Iodothyronine deiodinases (Dio) are selenocysteine-containing membrane enzymes that activate and inactivate the thyroid hormones (TH) through reductive iodide eliminations. The three deiodinase isoforms are homodimers sharing highly conserved amino acid sequences, but they differ in their regioselectivities for the deiodination reaction and regulatory features. Dios feature homologous transmembrane regions and catalytic domains with a catalytic selenocysteine (Sec) residue essential for their unique reductive deiodination mechanism. The Dio isoforms differ, however, in their regioselectivities: Dio1 can catalyze deiodination of both the inner (tyrosyl) and the outer (phenolic) ring, while Dio2 targets only the outer ring and Dio3 only the inner ring.

To explore the molecular basis of deiodinase isoform differences, we solved a crystal structure of the catalytic domain of Mus musculus Dio2 (mDio2cat; residues 71–262). The catalytic Sec130 was replaced with cysteine to simplify bacterial overexpression. Two lysine residues, Lys180-Lys181, were predicted as the best SER candidates based on sequence analyses with the SERp server and consistent with the structure of the homolog mDio3cat (likely surface position) and were thus mutated to Ala. The protein mDio2cat-(Lys180Ala-Lys181Ala; mDio2cat-AlaAla) indeed formed well-diffracting crystals and the structure of mDio2cat-AlaAla (from now on referred to as mDio2cat) could be solved and refined at a resolution of 1.1 Å to R/Rfree values of 14.5% and 16.9%, respectively. The mDio2cat structure comprises 183 residues, covering an N-terminal Gly as a cloning artifact, a small part of the linker to the transmembrane region (71–76), and the complete catalytic core (77–261), except for the C-terminal Arg262 and residues 94–102, which are not defined by electron density. All residues of the structure are within favored (96.5%) or allowed regions (2.9%) of the Ramachandran plot, except for Phe224, which is well defined by electron density. mDio2cat features a Trx/Prx fold with deiodinase-specific modifications and insertions and high similarity in the overall structure to mDio3cat, confirming the proposed conservation of a Trx/Prx-related fold among the Dio isoforms. The basic Trx fold provides β-strands β1–4, and the sheet they form is extended by a single strand, βD, from the deiodinase-specific insertion that further comprises an α-helix αD and the extended loop-D (residues 161–188), which protrudes out of the globular structure. A major difference between Dio2 and other isoforms, however, is a 15-residue (91–105) “Dio2-insertion” in the N-terminal region of the catalytic core. Interestingly, there is no electron density for nine central residues of the Dio2-insertion (94–102), indicating conformational heterogeneity or high flexibility.

> GAYKQVKLGEDAPNSSVVHVSNPESGNNYASEKTADGAECHLLDFASAERPLVVNFGSATCPPFTRQLPAFRQLVEEFSSVADFLLVYIDEAHPSDGWAVPGDSSLSFEVAAHRNQEDRCAAAHQLLERFSLPPQCQVVADRMDNNANVAYGVAFERVCIVQRRKIAYLGGKGPFSYNLQEVRSWLEKNFSKR1-(5-cyanopyrazin-2-yl)-3-isoquinolin-3-ylurea 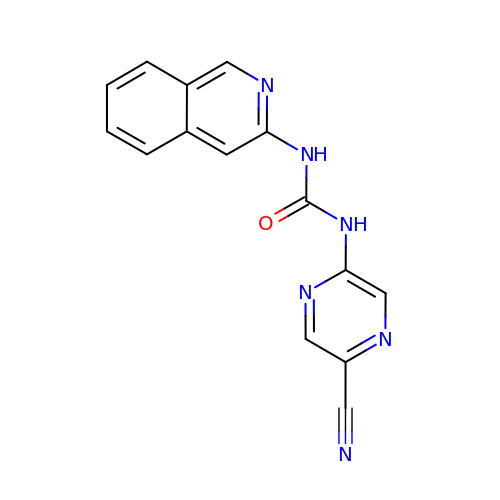| C15 H10 N6 O | GFPBJOCJVKFSBK-UHFFFAOYSA-N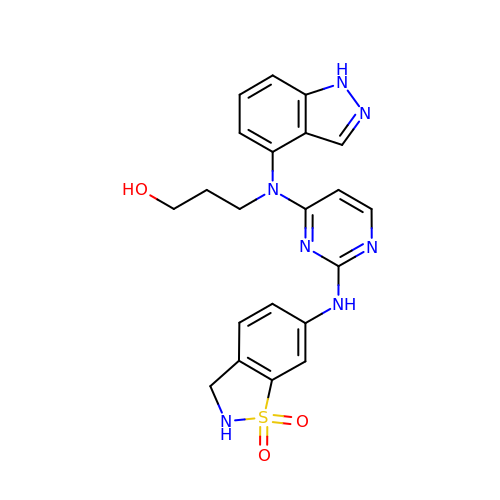3-[{2-[(1,1-dioxido-2,3-dihydro-1,2-benzothiazol-6-yl)amino]pyrimidin-4-yl}(1H-indazol-4-yl)amino]propan-1-ol | C21 H21 N7 O3 S | XIWBNOAYPAXNEG-UHFFFAOYSA-N[[(2~{R},3~{S},4~{R},5~{R})-5-(6-aminopurin-9-yl)-3,4-bis(oxidanyl)oxolan-2-yl]methoxy-oxidanyl-phosphoryl] 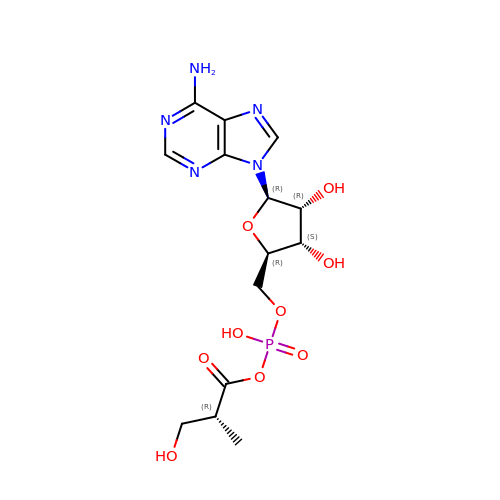(2~{R})-2-methyl-3-oxidanyl-propanoate | C14 H20 N5 O9 P | GTYNBQPSEMILMN-KWGHVAAJSA-N> ESVASHFALVTAYED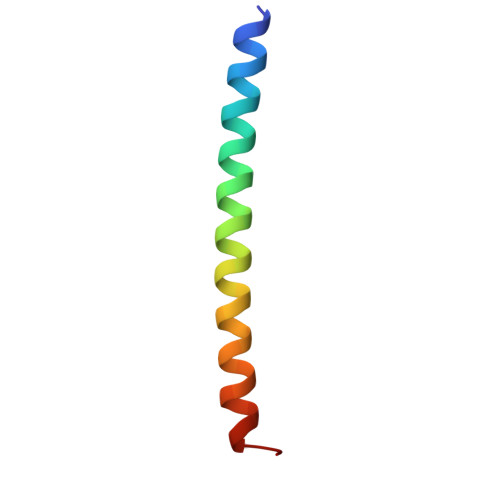IKKRLKDSEKENSLLKKRIRFLEEKLIA> AVSLDRTRAVFDGSEKSMTLDISNDNKQLPYLAQAWIENENQEKIITGPVIATPPVQRLEPGAKSMVRLSTTPDISKLPQDRESLFYFNLREIPPRSEKANVLQIALQTKIKLFYRPAAIKTRPNEVWQDQLILNKVSGGYRIENPTPYYVTVIGLGGSEKQAEEGEFETVMLSPRSEQTVKSANYNTPYLSYINDYGGRPVLSFICNGSRCSVKKEK;>APTIPQGQGKVTFNNTVVDAPCSISQKSADQSIDFGQLSKSFLEAGGVSKPMDLDIELV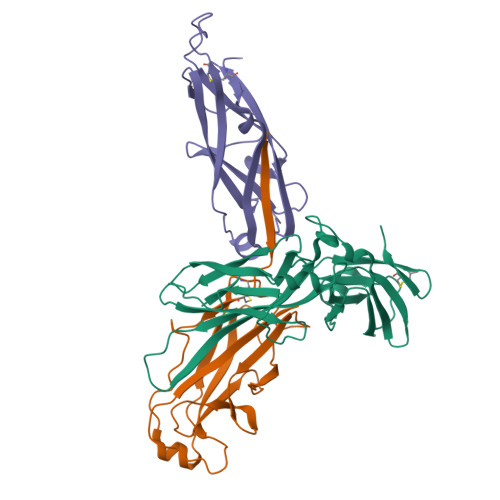NCDITAFKGGNGAKKGTVKLAFTGPIVNGHSDELDTNGGTGLAIVVQGAGKNVVFDGSEGDANTLKDGENVLHYTAVVKKSSAVGAAVTEGAFSAVANFNLTYQ[2x]> M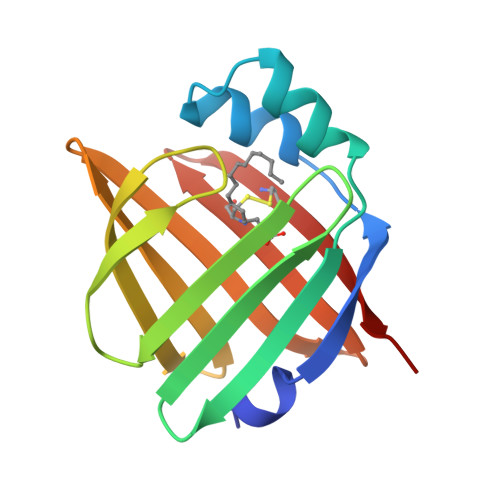ATVQQLEGRWRLVDSKGFDEYMKELGVGIALRKMGAMAKPDCIITCDGKNLTIKTESTLKTTQFSCTLGEKFEETTADGRKTQTVCNFTDGALVQHQEWDGKESTITRKLKDGKLVVECVMNNVTCTRIYEKVE2-(5-AMINO-6-OXO-2-PHENYL-6H-PYRIMIDIN-1-YL)-N-[2-(5-TERT-BUTYL-1,3,4-OXADIAZOL-2-YL)-1-(METHYLETHYL)-2-HYDROXYETHYL]ACETAMIDE 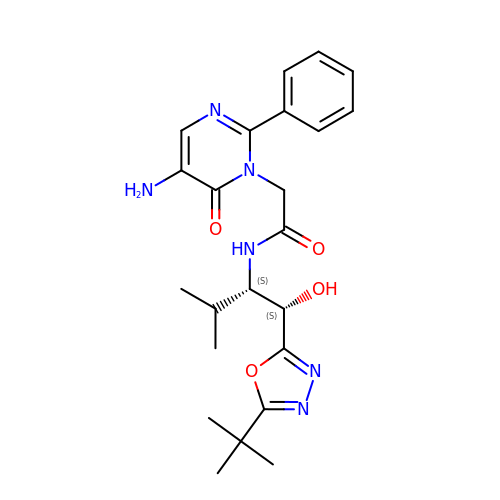| C23 H30 N6 O4 | HMPQTEPEMQZWQH-ROUUACIJSA-N>[2x]MTDSSSLRGVDADTEKRINVGKTHLQTLRNLETRCHDSLQALVVIDAGSSSTRTNVFLAKTRSCPNKGRSIDPDSIQLIREGKRFTGLRVVLEEWLDTYAGKDWESRPVDARLLFQYVPQMHEGAKKLMQLLEEDTVAILDSQLNEEQKVQVKALGIPVMLCSTAGV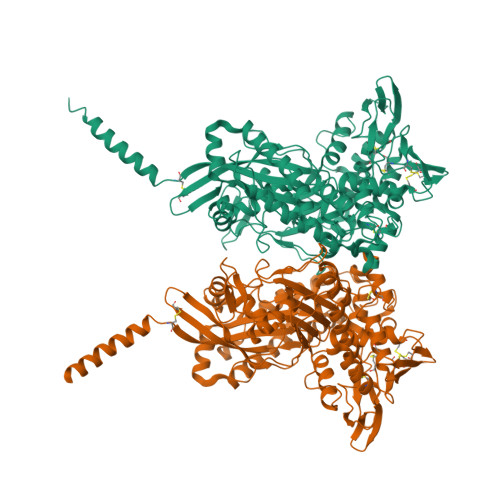RDFHEWYRDALFVLLRHLINNPSPAHGYKFFTNPFWTRPITGAEEGLFAFITLNHLSRRLGEDPARSMIDEYGVKHSRNDLAGVVEVGGASAQIVFPLQEGTVLPSSVRAVNLQRERLLPERYPSADVVSVSFMQLGMASSAGLFLKELCSNDEFLQGGICSNPCLFKGFQQSCSAGEVEVRPDGSASVNEDVRKNRLKPLATYCSVHNPEISFKVTNEMQCRENSIDPTKPLAERMKIENCSIIEGTGNFDKCVSQVESILVAPKLPLPANIEAASSGFESVDQVFRFASSTAPMFITGREMLASIDTLKDHRLLRSDFSGDVEELAEAAREFCSSEVIIRTDGPVIQLPNARGEQKLNSLNFDLCKTMALTVSLLRHMAAGENQPSFIKWEKSIAGPDGKPLADLGWQVGVILHHVLFTEEWGRTAYEAGYSHNLEHHHHHH>SPEALRIGYQKGSIGMVLAKSHQLLEKRYPESKISWVEFPAGPQMLEALNVGSIDLGSTGDIPPIFAQAAG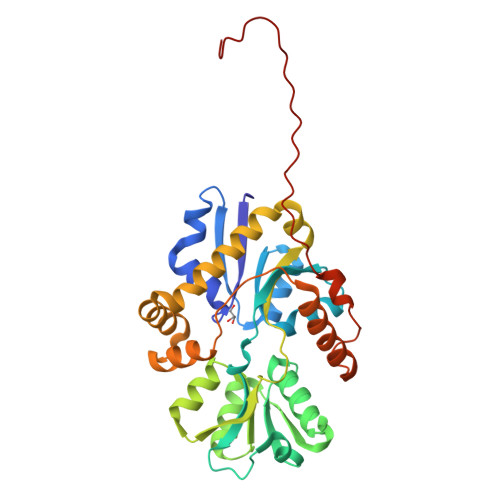ADLVYVGVEPPKPKAEVILVAENSPIKTVADLKGHKVAFQKGSSSHNLLLRALRQAGLKFTDIQPTYLTPADARAAFQQGNVDAWAIWDPYYSAALLQGGVRVLKDGTDLNQTGSFYLAARPYAEKNGAFIQGVLATFSEADALTRSQREQSIALLAKTMGLPAPVIASYLDHRPPTTIKPVNAEVAALQQQTADLFYENRLVPKKVDIRQRIWQPTQLEGKQLEFRVPGNENLYFQ[2x]(8E)-6,17,28-trihydroxy-1,6,12,17,23,28-hexaazacyclotritriacont-8-ene-2,5,13,16,24,27-hexone | C27 H46 N6 O9 | 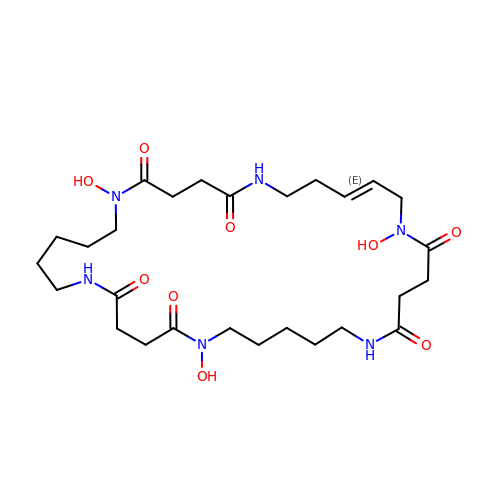SHTNNSLDUIEFSM-LREOWRDNSA-N(1S)-3-amino-4-[(2S)-1,1,1-trifluoro-3-oxopropan-2-yl]cyclopent-3-ene-1-carboxylic acid | C9 H10 F3 N O3 | 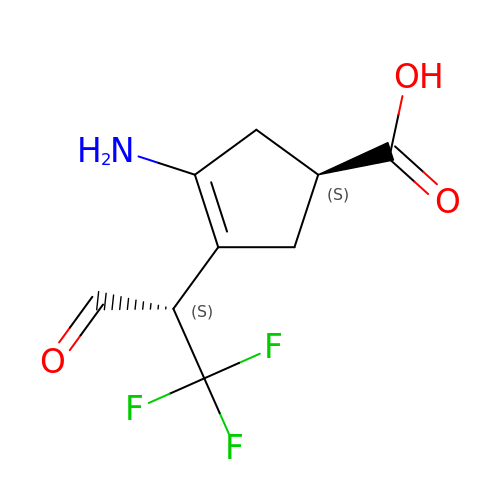FRXHJQNUUVTCON-UJURSFKZSA-N>GQSNMTNEMFDLAKLKSGVKNKRISSTDPTGGNRDHLEPFKPGEKRIIADIKGMGVINHIWVTIAPPPPTLSRNDIIIRMYWDGNDYPSVESPIGPFFGQGWDERYNYASLPLSAGPENGTGLSCYFAMPFEKGARIEIENQSDRNIDAFYFYVDYLEMAKLPKDMGRFHAWYNHNLTEALPEGETEWGVTGAQKPNTTGERNYVFMETQGKGHFVGINYYVHCPTPMWYGEGDDMWFIDGEKVPSLIGTGTEDFFNTAWCPKEAFSHPYFGYPRVNNDIGWLGRTHVYRFFIEDPIFFEKSLKGTIEHGSNNNLTLDLSTVAYWYQDSAVALPEAPT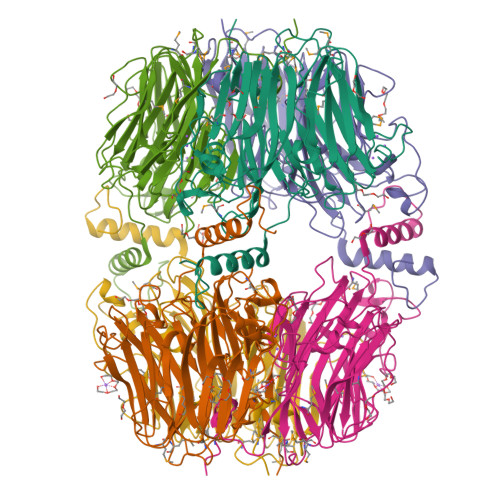KAQRAPKPFINHVDIHRWRDAWRKSKGNKATLWGNE[2x]>[2x]CTGVRFSDDEGNTYFGRNLDWSFSYGETILV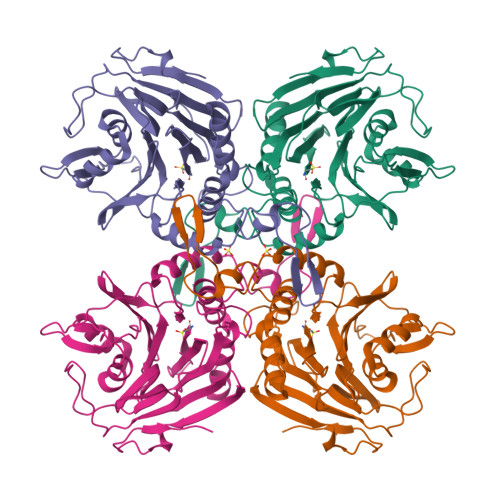TPRGYHYDTVFGAGGKAKPNAVIGVGVVMADRPMYFDCANEHGLAIAGLNFPGYASFVHEPVEGTENVATFEFPLWVARNFDSVDEVEETLRNVTLVSQIVPGQQESLLHWFIGDGKRSIVVEQMADGMHVHHDDVDVLTNQPTFDFHMENLRNYMCVSNEMAEPTSWGKASLTAWGAGVGMHGIPGDVSSPSRFVRVAYTNAHYPQQNDEAANVSRLFHTLGSVQMVDGMAKMGDGQFERTLFTSGYSSKTNTYYMNTYDDPAIRSYAMADYDMDSSELISVAR>[4x]MGSSHHHHHHSQDPMSTGTFVVSQPLNYRGGARVEPADASGTEKAFEPATGRVIATFTCSGEKEVNLAVQNAKAAFKIWSQKSGMERCRILLEAARIIREREDEIATMECINNGKSIFEARLDIDISWQCLEYYAGLAASMAGEHIQLPGGSFGYTRREPLGVCVGIGAWNYPFQIASWKSAPALACGNAMVFKPSPFTPVSALLLAEIYSEAGVPPGLFNVVQGGAATGQFLCQHPDVAKVSFTGSVPTGMKIMEMSAKGIKPVTLELGGKSPLIIFSDCDMNNAVKGALMANFLTQGQVCCNGTRVFVQKEILDKFTEEVVKQTQRIKIGDPLLEDT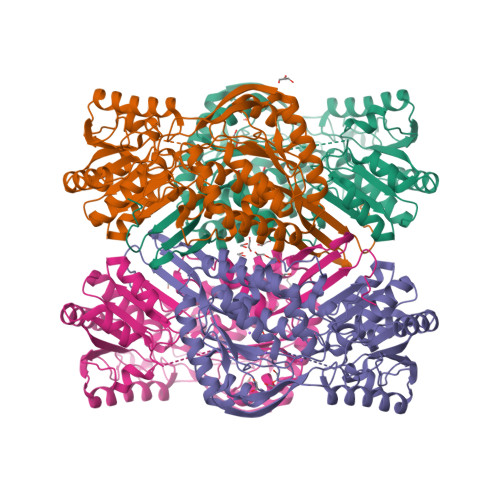RMGPLINRPHLERVLGFVKVAKEQGAKVLCGGDIYVPEDPKLKDGYYMRPCVLTNCRDDMTCVKEEIFGPVMSILSFDTEAEVLERANDTTFGLAAGVFTRDIQRAHRVVAELQAGTCFINNYNVSPVELPFGGYKKSGFGRENGRVTIEYYSQLKTVCVEMGDVESAF> QETPAEIDPSKIPGEWRIIYAAADNKDKIVEGGPLRNYYRRIECINDCESLSITFYLKDQGTCLLLTEVAKRQEGYVYVLEFYGTNTLEVIHVSENMLVTYVENYDGERITKMTEGLAKGTSFTPEELEKYQQLNSERGVPNENIENLIKTDNCPP

Lipocalins are typically small proteins (about 200 amino acid residues) composed of an 8-stranded up-and-down antiparallel β-barrel and one α-helix. There is a hydrophobic cavity inside the β-barrel capable of binding a hydrophobic or amphiphilic ligand. Bos d 2 contains a central β-barrel composing of eight antiparallel β-strands (A-H). In addition, there is a short β-strand (I) as well as an α-helix.

Because the protein had been crystallised at an acidic pH (3.4–4.5), we decided to search for a new crystal form at a more neutral pH. The search for new crystal forms for bovine allergen Bos d 2 at neutral pH resulted in two new crystal forms. Trigonal crystals diffracted at 1.75 Å resolution. Again, the asymmetric unit contained one Bos d 2 molecule and a dimer can be formed with the use of a crystallographic symmetry operator. The interface area between monomers in the trigonal crystal is also 389 Å2 but there are many more hydrophobic contacts on the monomer-monomer interface. The side-chains of Thr62, Leu64 and Leu66 from the β-strand D form the core of the interface. In addition, the residues Phe82 and Tyr83 from the L5 loop, as well as Leu57 from the β-strand C, are located on the interface. Because there is a clearly higher number of hydrophobic residues on this interface, we assume that this interface is more favourable in solution than the dimer observed in monoclinic crystal form. Dimerization of Bos d 2 and Per a 4 resemble each other: both lipocalins form an extended β-sheet through β-strand D, although there are also some differences in the packing of these β-strands. When the protein concentration was increased to 90 μM, the relative intensity of the dimer increased accordingly. These results indicate that rBos d 2 is indeed a weak transient dimer in solution.> MSNRLIFDADWLVPEQVQVAGQAIQYYAARNIQYVQHPVAAIQVLNVFVPAAYLHGSSVNGYQRATAPILMPNTVGGYLPGPADDPQRVTWPTNAGTIQQALKRGYVVVAAGIRGRTTVDKSGQRVGQAPAFIVDMKAAI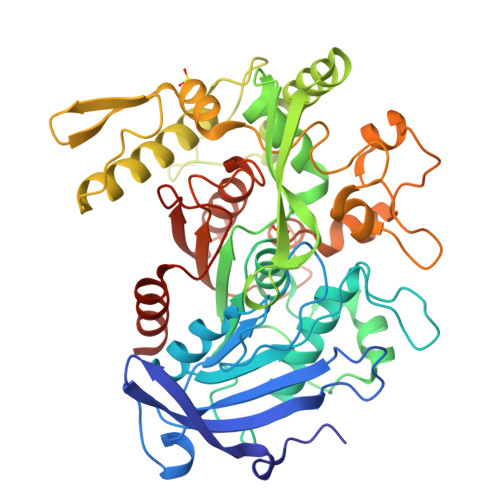RYVKYNQGRLPGDTNRIITNGTSAGGATSALAGASGNSAYFEPALTALGAAPATDDIFAVSAYCPIHNLEHADMAYEWQFNGINDWHRYQPVAGTTKNGRPKFEPVSGQLTVEEQALSLALKAQFSTYLNQLQLTASDGTHLTLNEAGMGSFRDVVRQLLISSAQTAFDQGTDIHKYAGFVVTGNQVTDLDLSAYLKSLTRMKAVPAFDQLDLTSPENNLFGDATAKAKHFTALAQTRSTVTAQLADAELIQAINPLSYLTTTSSQVAKHWRIRHGAADRDTSFAIPIILAIMLENHGYGIDFALPWDIPHSGDYDLGDLFSWIDGLCQLEHHHHHH D-mannose | C6 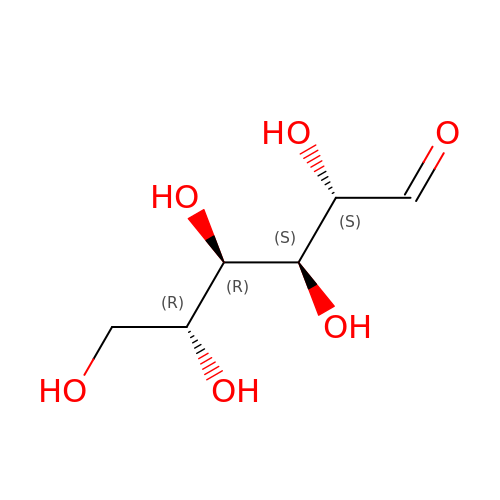H12 O6 | GZCGUPFRVQAUEE-KVTDHHQDSA-N Among them, the Par (partitioning defective) complex, the first set of genes identified in polarization of Caenorhabditis elegans embryos during development, are evolutionarily conserved master polarity determinants from worms to mammals. The Par complex plays indispensable roles in diverse polarity-related contexts, such as asymmetric cell division (ACD), establishment of apical–basal polarity in epithelial cells, oriented cell migration, and neuronal polarization. Par3 has three PDZ (PSD-95, DLG, and ZO-1) domains that mediate protein–protein interactions. Mammalian Par3 PDZ3 specifically recognizes Par6 PBM, and the Par3/Par6 interaction can be significantly enhanced by Par3 NTD and Par6 PB1 through their oligomerization.

The crystal structure of Par3 PDZ3 in complex with a Par6β PBM peptide revealed that the last three residues of Par6β PBM (−2ITL0) binds to the αB–βB groove of PDZ3 using a classical PDZ binding mode. The carboxyl terminal of L(0) from Par6β PBM forms extensive hydrogen bonds with the canonical “G600LG602F” loop of Par3 PDZ3. The sidechain of I(−2) from Par6β PBM inserts into a shallow hydrophobic pocket formed by the αB–βB groove of Par3 PDZ3. In line with the structure, the G600,602 A mutation of Par3 PDZ3 dramatically weakened the PDZ3–PBM interaction ~20-fold. We further found that addition of 1,6-hexanediol impaired the hydrophobic interaction between Par3 PDZ3 and Par6β PBM. Overall, Par3N specifically binds to Par6β via the PDZ3–PBM recognition, and both Par3 NTD and Par6β PB1 enhance the interaction likely through oligomerization-induced avidity increase. As a key driving factor for the specific interaction and LLPS of Par3N and Par6β, Par6β PBM is completely conserved in Par6γ but varies in Par6α. As expected, Par6γ PBM but not Par6α PBM bound to Par3 PDZ3 equally well as that of Par6β PBM. We then constructed a Par6α chimera mutant, with its PBM replaced by the Par6β PBM, and the puncta formation property was gained in cells co-expressed with Par3N and the Par6α chimera, further demonstrating the critical role of PBM–PDZ3 recognition in promoting puncta formation of Par3N in living cells. Par6β promotes Par3N LLPS, relying on the specific interaction between Par3 PDZ3 and Par6β PBM, as well as the high valency of both proteins.

> LEEDGTIITL;> GPGSEFGTREFLTFEVPLNDSGSAGLGVSVKGNRSKENHADLGIFVKSIINGGAASKDGRLRVNDQLIAVNGESLLGKANQEAMETLRRSMSTEGNKRGMIQLIVARRIS> QFAKPEDAVKYRQSAFTLMASHFGRMTPVVKGQAPYDAAQIKANVEVLKTLSALPWAAFGPGTEGGDARPEIWSDAASFKQKQQAFQDNIVKLSAAADAGDLDKLRAAFGDVGASCKACHDAYRK

Cytochromes c′ occur in methanotrophic, denitrifying and photosynthetic bacteria and have proposed roles in protection against nitrosative stress, NO trafficking during denitrification or pathogen defence. All cytochromes c′ have a 4 α-helix bundle structure containing a heme centre with a solvent exposed proximal His ligand and a buried hydrophobic distal pocket with a non-coordinated residue (Leu or Phe, rarely Met or Tyr) in a position to exert steric influence on the binding of diatomic gases. Unusually, cytochromes c′ are able to utilize both heme faces (distal and proximal) as a means of discriminating NO from other diatomic gases. In order to understand the factors controlling distal versus proximal NO coordination, we have examined NO binding to AXCP variants in which the occluding distal residue Leu16 is replaced with residues that are smaller (Ala, Val), of comparable size (Ile) or larger (Phe).

Kinetic data confirm that this variant has a high degree of distal steric constraint that destabilizes distal heme–NO binding (vide infra).Mislocalization, cleavage, and aggregation of the human protein TDP-43 is found in many neurodegenerative diseases. TDP-43 protein has several functions, and its modular structure facilitates this multitasking. Two centrally located RNA recognition motifs (RRM) strongly bind UG-rich RNA (Lukavsky et al., 2013) or TG-rich DNA (Austin et al., 2014) directing TDP-43 to pre-mRNAs and intronic sites (Tollervey et al., 2011). At the N terminus, a ubiquitin or dix-like domain (Mompeán et al., 2016, Qin et al., 2014) provides a polymerization surface that enables formation of dimer and higher-order oligomers predominantly found in the cell nucleus (Afroz et al., 2017).

A fragment of TDP-43 comprising residues 1-270 including NTD and RRMs was used in crystallization experiments and the structure of the NTD (residues 1-80) was elucidated at 2.55 Å resolution. The protein appears to have been auto-cleaved at N terminal to RRM2 during the 7 days required for crystallization to produce diffraction-quality crystals, whereas RRM1 is conformationally mobile in crystallo and therefore not visible. The TDP-43 NTD crystallized in space group P212121 with five identical molecules in the asymmetric unit. The NTD adopts a similar conformation as reported in a recent crystallographic structure obtained in P63 space group (Afroz et al., 2017). The head-to-tail interfaces between the molecules differ from those reported previously (Afroz et al., 2017). A sulfate ion binds at the interface between the molecules and is bonded to Arg52 and Arg55, which serves as a wedge, increasing the distance between the monomers. This binding of a sulfate ion to Arg52 and Arg55 rearranges their side chains preventing strong bonding between Arg52-Glu3 and Arg55-Glu21 reported in an earlier NTD structure (Afroz et al., 2017). The changes in the position of the monomers against each other alter the superhelical bundle arrangement observed previously (Afroz et al., 2017). Each spiral, with radius of 46 Å, has 10 NTD molecules in a full turn with distance between two rings being ~36 Å. Analysis of the structural changes on sulfate binding confirms that ligand binding at the molecular interface could change the nature of the helical arrangements. These head-to-tail interactions that lead to parallel spirals are consistent with the view that physiological TDP-43 oligomerization is mediated by its NTD and may be key to prevent the formation of pathologic aggregates.

>MSEYIRVTEDENDEPIEIPSEDDGTVLLSTVTAQFPGACGLRYRNPVSQCMRGVRLVEGILHAPDAGWGNLVYVVNYPKD[5x]> TMGGDALRVPFLDFATATPKRHQTVVPGVGTLHDCCEHSPLFSAVARRLLFNSLVPAQLKGRDFGGDHTAKLEFLAPELVRAVARLRFKECAPADVVPQRNAYYSVLNTFQALHRSEAFRQLVHFVRDFAQLLKTSFRASSLTETTGPPKKRAKVDVATHGRTYGTLELFQKMILMHATYFLAAVLLGDHAEQVNTFLRLVFEIPLFSDAAVRH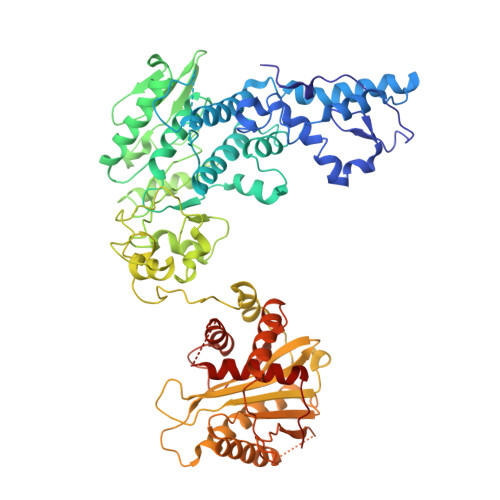FRQRATVFLVPRRHGKTWFLVPLIALSLASFRGIKIGYTAHIRKATEPVFEEIDACLRGWFGSARVDHVKGETISFSFPDGSRSTIVFASSHNTNGIRGQDFNLLFVDEANFIRPDAVQTIMGFLNQANCKIIFVSSTNTGKASTSFLYNLRGAADELLNVVTYICDDHMPRVVTHTNATACSCYILNKPVFITMDGAVRRTADLFLADSFMQEIIGGQARETGDDRPVLTKSAGERFLLYRPSTTTNSGLMAPDLYVYVDPAFTANTRASGTGVAVVGRYRDDYIIFALEHFFLRALTGSAPADIARCVVHSLTQVLALHPGAFRGVRVAVEGNSSQDSAVAIATHVHTEMHRLLASEGADAGSGPELLFYHCEPPGSAVLYPFFLLNKQKTPAFEHFIKKFNSGGVMASQEIVSATVRLQTDPVEYLLEQLNNLTETVSPNTDVRTYSGKRNGASDDLMVAVIMAIYLAAQAGPPHTF In Saccharomyces cerevisiae, reduced potassium dependency-3 (Rpd3) resides in two distinct histone deacetylase complexes, termed Rpd3S and Rpd3L1–3. The Rpd3S complex functions to repress transcriptional initiation within the coding region of genes during RNA polymerase II elongation by maintaining hypoacetylation. Rco1 recognizes unmodified H3K4 (H3K4me0) via its PHD1 domain and associates with Eaf3 to enhance the Eaf3–H3K36me3 interaction. In this study, we presented the structures of Eaf3MRG bound with Rco1PHD1–SID and H3K4me0 or with a fragment of Eaf7.

To gain mechanistic insights into the Eaf3–Rco1 interaction and the preference of Rco1 for H3K4me0, we solved the complex structure of Eaf3MRG–Rco1PHD1–SID–H3K4me01–12 at 1.60 Å resolution. In the ternary complex, Eaf3MRG adopts a canonical fold similar to that of MRG15MRG, and buries an area of approximately 2072 Å2 with Rco1PHD1–SID. Rco1PHD1–SID interacts with Eaf3MRG via three interfaces, with two for SID (interfaces I and II) and one for PHD1 (interface III). The Rco1SID C-terminal region contacts α1, α3, and α5 of Eaf3MRG, with the loop between α3 and α4 interacting with Eaf3MRG via hydrophobic and hydrogen bonding interactions. α3 of Rco1SID further makes hydrophobic interactions with α3, α5, and α6 of Eaf3MRG. Unexpectedly, Rco1PHD1 also interacts with α3, η1, α4, and α8 of Eaf3MRG via electrostatic and hydrophobic interactions, albeit fewer than those found between Rco1SID and Eaf3MRG. The interactions between Eaf3MRG and Rco1PHD1 raise the possibility that Eaf3MRG allosterically reinforces the Rco1–H3 interaction by stabilizing Rco1PHD1. Consistently, ITC binding assays demonstrated that the Eaf3–Rco1 complex binds to the H3K4me0 peptide with 5-fold higher affinity than Rco1PHD1 alone (KD values: 22 μM vs 110 μM), underscoring the Eaf3MRG–Rco1PHD1 interaction mediated by Arg300 and Arg303 of Eaf3MRG. Similar to previously reported PHD complex structures, the H3K4me0 peptide lies in the negative surface of Rco1PHD1 by forming a two-stranded antiparallel β-sheet with Rco1PHD1 β1. Collectively, the first five residues of the H3K4me0 peptide are specifically recognized by Rco1PHD1.

> PKISLQIPIKLKSVLVDDWEYVTKDKKICRLPADVTVEMVLNKYEHEVSQELESPGSQSQLSEYCAGLKLYFDKCLGNMLLYRLERLQYDELLKKSSKDQKPLVPIRIYGAIHLLRLISVLPELISSTTMDLQSCQLLIKQTEDFLVWLLMHVDEYFNDKDPNRSDDALYVNTSSQYEGVALG;> ENEDFCSACNQSGSFLCCDTCPKSFHFLCLDPPIDPNNLPKGDWHCNECKFKIFINNSMATLKKIESNFIKQNNNVKIFAKLLFNIDSHNPKQFQLPNYIKETFPAVKTGSRGQYSDE;> ARTKQT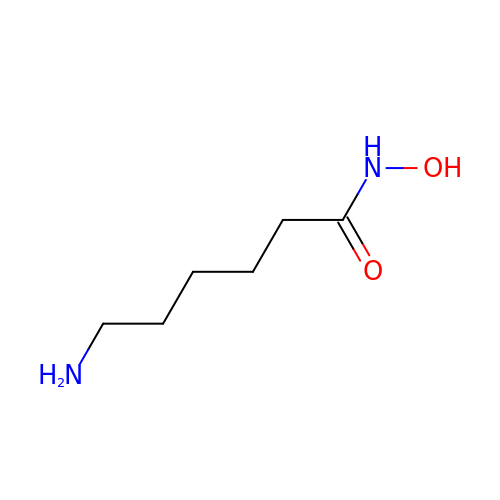6-amino-N-hydroxyhexanamide | C6 H14 N2 O2 | HAQVDFULTKFINY-UHFFFAOYSA-N> MGAQVTRQQTGTHENANVATNGSHITYNQINFY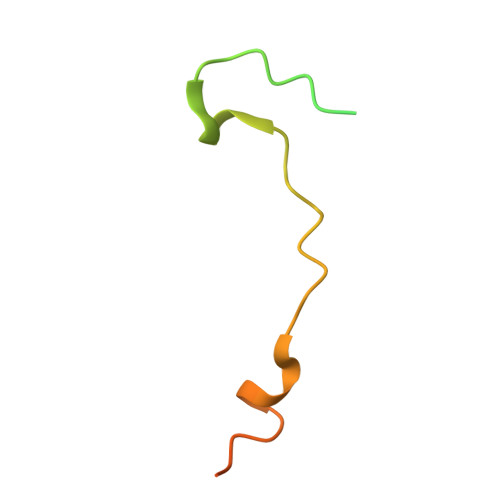KDSYAASASKQDFSQDPSKFTEPVVEGLKAGAPVLK>GUTTTGXCAAAAC[4x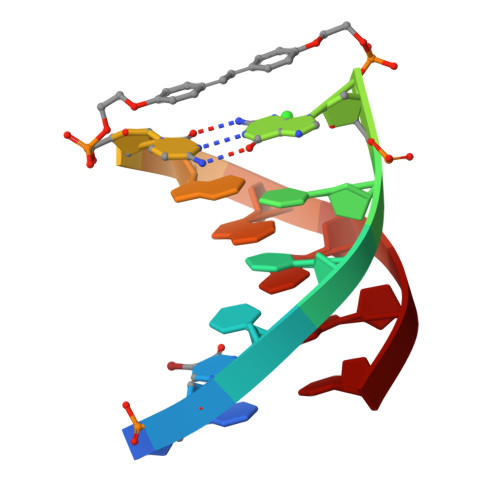]> APADRLKALVDAAVQPVMKANDIPGLAVAISLKGEPHYFSYGLASKEDGRRVTPETLFEIGSVSKTFTATLAGYALTQDKMRLDDRASQHWPALQGSRFDGISLLDLATYTAGGLPLQFPDSVQKDQAQIRDYYRQWQPTYAPGSQRLYSNPSIGLFGYLAARSLGQPFERLMEQQVFPALGLEQTHLDVPEAALAQYAQGYGKDDRPLRVGPGPLDAEGYGVKTSAADLLRFVDANLHPERLDRPWAQALDATHRGYYKVGD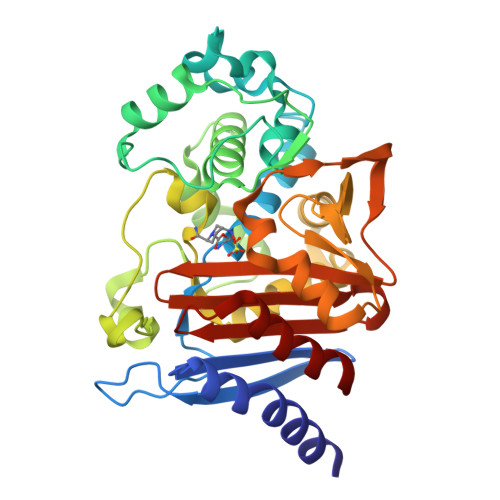MTQGLGWEAYDWPISLKRLQAGNSTPMALQPHRIARLPAPQALEGQRLLNKTGSTNGFGAYVAFVPGRDLGLVILANRNYPNAERVKIAYAILSGL> MKKLKKMEQNKTAATRYRQKKRAEQEALTGECKELEKKNEALKERADSLAKEIQYLKDLIEEV;> MEYKMRRERNNIAVRKSRDKAKMRNLETQHKVLEL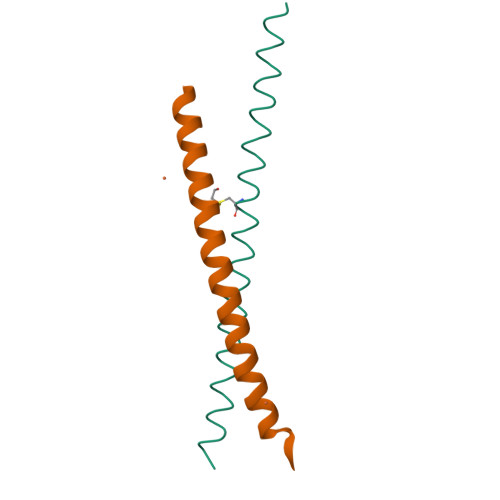TAENERLQKKVEQLSRELSTLRNLFKQL> 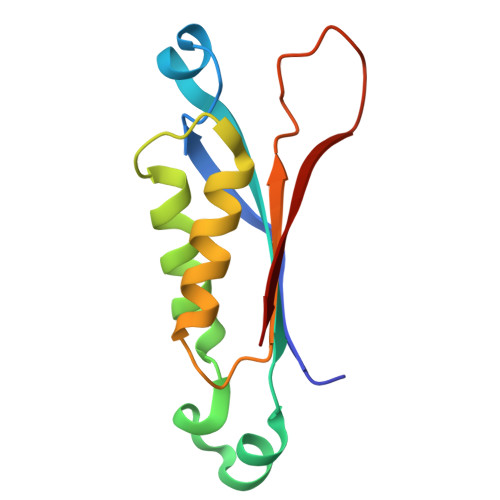MADRIELRGLTVHGRHGVAAHERVAGQRFVIDVTVWIDLAEAANSDDLADTYDYVRLASRAAEIVAGPPRKLIETVGAEIADHVMDDQRVHAVEVAVHKPQAPIPQTFDDVAVVIRRSR> GHMQIGWRREGIKYRRNELFLDVLESVNLLMSPQGQVLSAHVSGRVVMKSYLSGMPECKFGMNDKIVIEKQGKGTADETSKSGKQ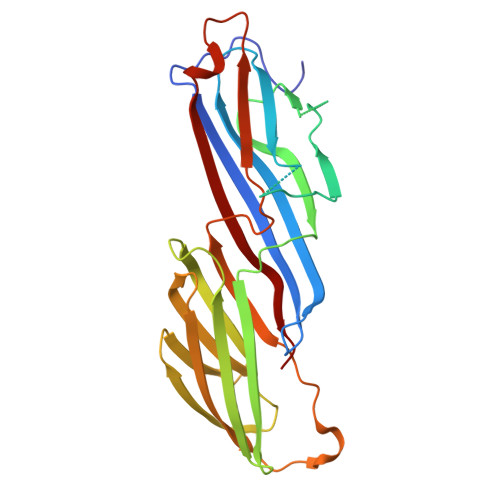SIAIDDCTFHQCVRLSKFDSERSISFIPPDGEFELMRYRTTKDIILPFRVIPLVREVGRTKLEVKVVIKSNFKPSLLAQKIEVRIPTPLNTSGVQVICMKGKAKYKASENAIVWKIKRMAGMKESQISAEIELLPTNDKKKWARPPISMNFEVPFAPSGLKVRYLKVFEPKLNYSDHDVIKWVRYIGRSGIYETRC> NECLGTIGPVTPLDAS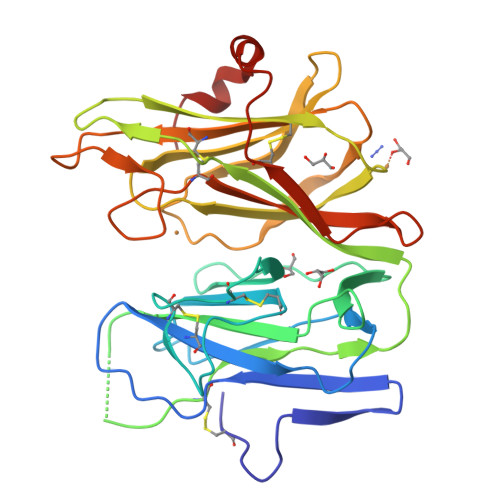DFALDIRMPGVTPKESDTYFCMSMRLPVDEEAFVIDFKPRASMDTVAHMLLFGCNMPSSTGSYWFCDEGTCTDKANILYAWARNAPPTRLPKGVGFRVGGETGSKYFVLQVHYGDISAFRDNHKDCSGVSVHLTRVPQPLIAGMYLMMSVDTVIPPGEKVVNADISCQYKMYPMHVFAYRVHTHHLGKVVSGYRVRNGQWTLIGRQNPQLPQAFYPVEHPVDVTFGDILAARCVFTGEGRTEATHIGGTSSDEMCNLYIMYYMEAKYALSFMTCTKNVAPDMFRTIPAEANIPIPV>MTNMTQASATERKGASDLLRFKIFGMPLPLYAFALITLLLSHFYNAIPTDLVGGFALMFVMGAIFGEIGKRLPIFNKYIGGAPVMIFLVAAYFVYAGIFTQKEIDAISNVMDKSNFLNLFIAVLITGAILSVNRKLLLKSLLGYIPTILAGIVGASLFGIVIGLCFGIPVDRIMMLYVLPIMGGGNGAGAVPLSEIYHSVTGRSREEYYSTAIAILTIANIFAIIFAALLDMVGKKYTWLSGEGELVRKASFKTEDDEKAG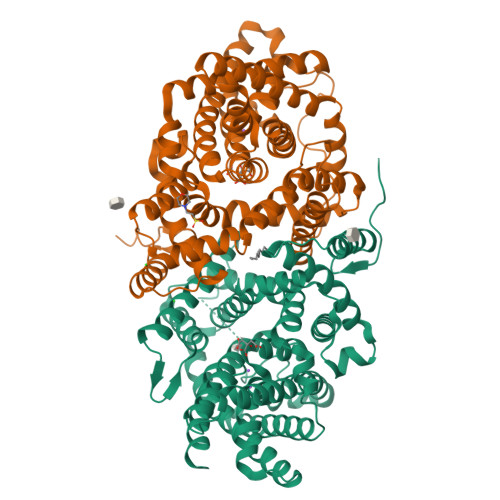QITHRETAVGMVLSTTCFLLAYVVAKKILPSIGGVSIHYFAWMVLIVAALNASGLCSPEIKAGAKRLSDFFSKQLLWVLMVGVGVCYTDLQEIIDALTFANVVIAAIIVVGAVVGAAIGGWLIGFYPIESSITAGLCMANRGGSGDLEVLSACNRMNLISYAQISSRLGGGIVLVIASIVFSMMVLE[4x]>[2x]MDVVVRLPDVAVPGEAVQASARQAVIHLVDIAGITSSTPADYATKNLYLWNNETCDALSAPVADWNDVSTTPTGSDKYGPYWVIPLTKESGCINVIVRDGTNKLIDSDLRVSFSDFTDRTVSVIAGNSAVYDSRADAFRAAFGVALADAHWVDKTTLLWPGGENKPIVRLYYSHSSKVAADSNGEFSDKYVKLTPTTVSQQVSMRFPHLASYPAFKLPDDVNVDELLQGETVAIAAESDGILSSATQVQTAGVLDDTYAAAAEALSYGAQLTDSGVTFRVWAPTAQQVELVIYSADKKVIASHPMTRDSASGAWSWQGGSDLKGAFYRYAMTVYHPQSRKVEQYEVTDPYAHSLSTNSEYSQVVDLNDSALKPEGWDGLTMPHAQKTKADLAKMTIHESHIRDLSAWDQTVPAELRGKYLALTAQESNMVQHLKQLSASGVTHIELLPVFDLATVNE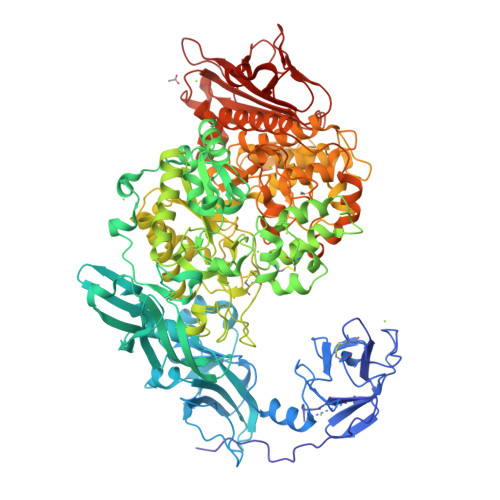FSDKVADIQQPFSRLCEVNSAVKSSEFAGYCDSGSTVEEVLTQLKQNDSKDNPQVQALNTLVAQTDSYNWGYDPFHYTVPEGSYATDPEGTARIKEFRTMIQAIKQDLGMNVIMDVVYNHTNAAGPTDRTSVLDKIVPWYYQRLNETTGSVESATCCSDSAPEHRMFAKLIADSLAVWTTDYKIDGFRFDLMGYHPKAQILSAWERIKALNPDIYFFGEGWDSNQSDRFEIASQINLKGTGIGTFSDRLRDAVRGGGPFDSGDALRQNQGVGSGAGVLPNELTTLSDDQARHLADLTRLGMAGNLADFVLIDKDGAVKRGSEIDYNGAPGGYAADPTEVVNYVSKHDNQTLWDMISYKAAQEADLDTRVRMQAVSLATVMLGQGIAFDQQGSELLRSKSFTRDSYDSGDWFNRVDYSLQDNNYNVGMPRSSDDGSNYDIIARVKDAVATPGETELKQMTAFYQELTALRKSSPLFTLGDGATVMKRVDFRNTGADQQTGLLVMTIDDGMQAGASLDSRVDGIVVAINAAPESRTLQDFAGTSLQLSAIQQAAGDRSLASGVQVAADGSVTLPAWSVAVLELPQGESQGAGLPVSSK>MAEQVALSRTQVCGILREELFQGDAFHQSDTHIFIIMGASGDLAKKKIYPTIWWLFRDGLLPENTFIVGYARSRLTVADIRKQSEPFFKATPEEKLKLEDFFARNSYVAGQYDDAASYQRLNSHMNALHLGSQANRLFYLALPPTVYEAVTKNIHESCMSQIGWNRIIVEKPFGRDLQSSDRLSNHISSLFREDQIYRIDHYLGKEMVQNLMVLRFANRIFGPIWNRDNIACVILTFKEPFGTEGRGGYFDEFGIIRDVMQNHLLQMLCLVAMEKPASTNSDDVRDEKVKVLKCISEVQANNVVLGQYVGNPDGEGEATKGYLDDPTVPRGSTTATFAAVVLYVENERWDGVPFILRCGKALNERKAEVRLQFHDVAGDIFHQQCKRNELVIRVQPNEAVYTKM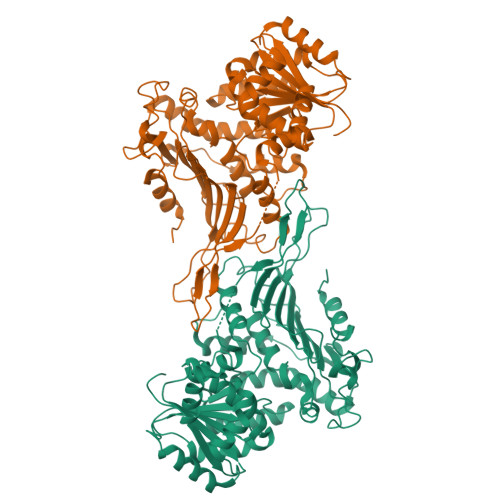MTKKPGMFFNPEESELDLTYGNRYKNVKLPDAYERLILDVFCGSQMHFVRSDELREAWRIFTPLLHQIELEKPKPIPYIYGSRGPTEADELMKRVGFQYEGTYKWVNPHKL[2x]> GSHMWDAQFENLLRRYLPFLSADQPLEQDINLRDIGLDSLGTVELLSELENTYDVHFQDEALTKETFE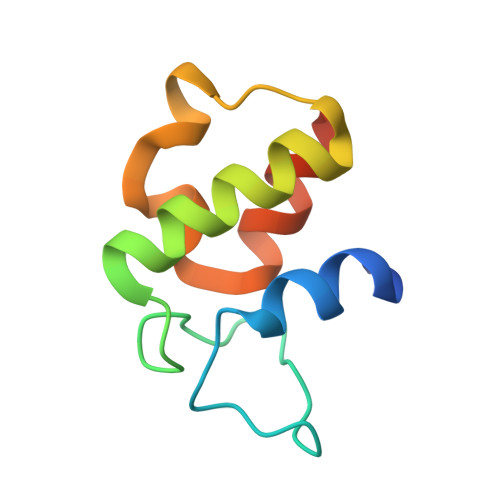TPGVLWKTLSQMVEPRH> GSHMATYYSNDFRAGLKIMLDGEPYAVEASEFVKPGKGQAFARVKLRRLLTGTRVEKTFKSTDSAEGADVVDMNLTYLYNDGEFWHFMNNETFEQLSADAKAIGDNAKWLLDQAECIVTLWNGQPISVT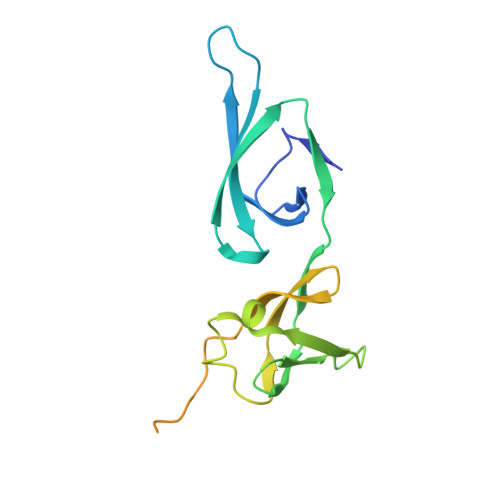PPNFVELEIVDTDPGLKGDTAGTGGKPATLSTGAVVKVPLFVQIGEVIKVDTRSGEYVSRVK> MAISLATKAATDALKVNRAPVGVEPQEVHKWLQSFNWDFKENRTKYPTKYHMANETKEQFKVIAKEYARMEAAKDERQFGTLLDGLTRLGAGNKVHPRWGETMKVISNFLEVGEYNAIAASAMLWDSATAAEQKNGYLAQVLDEIRHTHQ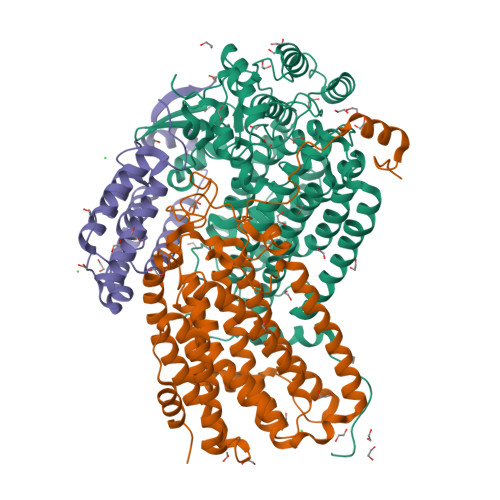CAFINHYYSKHYHDPAGHNDARRTRAIGPLWKGMKRVFADGFISGDAVECSVNLQLVGEACFTNPLIVAVTEWASANGDEITPTVFLSVETDELRHMANGYQTVVSIANDPASAKFLNTDLNNAFWTQQKYFTPVLGYLFEYGSKFKVEPWVKTWNRWVYEDWGGIWIGRLGKYGVESPASLRDAKRDAYWAHHDLALAAYAMWPLGFARLALPDEEDQAWFEANYPGWADHYGKIFNEWKKLGYEDPKSGFIPYQWLLANGHDVYIDRVSQVPFIPSLAKGTGSLRVHEFNGKKHSLTDDWGERQWLIEPERYECHNVFEQYEGRELSEVIAEGHGVRSDGKTLIAQPHTRGDNLWTLEDIKRAGCVFPDPLAKF;> MSQPQSSQVTKRGLTDPERAAIIAAAVPDHALDTQRKYHYFIQPRWKRLSEYEQLSCYAQPNPDWIAGGLDWGDWTQKFHGGRPSWGNESTELRTTDWYRHRDPARRWHHPYVKDKSEEARYTQRFLAAYSSEGSIRTIDPYWRDEILNKYFGALLYSEYGLFNAHSSVGRDCLSDTIRQTAVFAALDKVDNAQMIQMERLFIAKLVPGFDASTDVPKKIWTTDPIYSGARATVQEIWQGVQDWNEILWAGHAVYDATFGQFARREFFQRLATVYGDTLTPFFTAQSQTYFQTTRGAIDDLFVYCLANDSEFGAHNRTFLNAWTEHYLASSVAALKDFVGLYAKVEKVAGATDRAGVSEALQRVFGDWKIDYADKIGFRVDVDQKVDAVLAGYKN;> MAKREPIHDNSIRTEWEAKIAKLTSVDQATKFIQDFRLAYTSPFRKSYDIDVDYQYIERKIEEKLSVLKTEKLPVADLITKATTGEDAAAVEATWIAKIKAAKSKYEAERIHIEFRQLYKPPVLPVNVFLRTDAALGTVLMEIRNTDYYGTPLEGLRKERGVKVLHLQA>[2x]WDGKADGTGTHAMIATQGVTILENDLSSNEPEVIRNNLEILKQNMHDLQLGSTYPDYDKNAYDLYQDHFWDPDTDNNFTKDSKWYLSYSIPDTAESQIRKFSALARYEWKRGNYKQATFYLGEAMHYFGDADTPYHAANVTAVDSPGHVKFETFAEDRKDQYKINTTGSKTNDAFYSNILTNEDFNSWSKEFARSFAKTAKDLYYSHANMSCSWDEWDYAAKVALANSQKGTSGYIYRF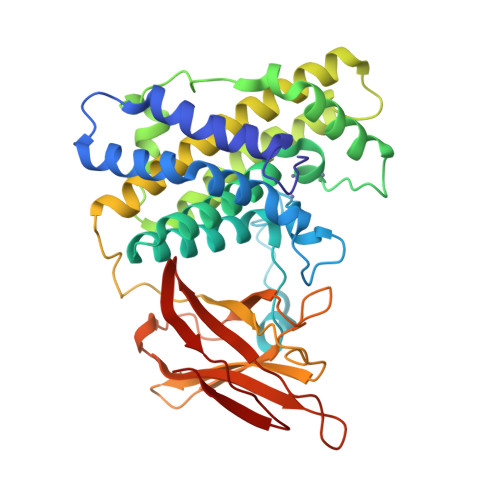LHDVSDGKDSSANKNVNELVAYITTGGEKYAGTDDYMYFGIKTKDGQTQEWTMDNPGNDFMTGSQDTYTFKLKDKNLKIDDIQNMWIRKSKYTEFGDDYKPANIKVIANGNVVLNKDINEWISGNSTYNIK> A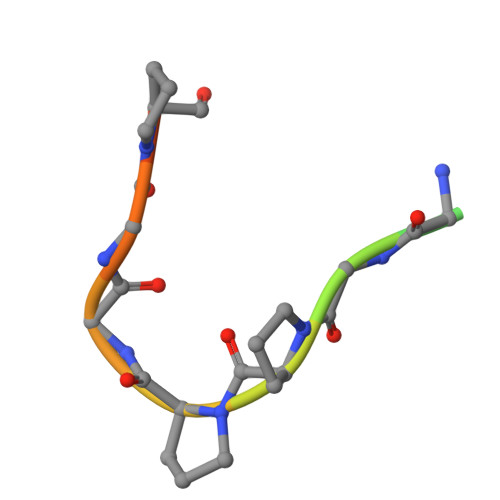YTVVGGPPGGPPVR> MASHHHHHHGSMAEGEEYDKILVLNFGSQYFHLIVKRLNNIKIFSETKDYGVELKDIKDMNIKGVILSGGPYSVTEAGSPHLKKEVFEYFLEKKIPIFGIAYGMQEIAVQMNGEVKKSKTSEYGCTDVNILRNDNINNITYCRNFGDSSSAMDL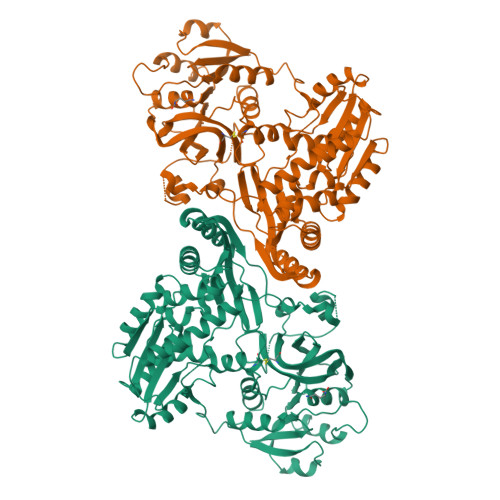YSNYKLMNETCCLFENIKSDITTVWMNHNDEVTKIPENFYLVSSSENCLICSIYNKEYNIYGVQYHPEVYESLDGELMFYNFAYNICKCKKQFDPIRYHELELKNIEKYKHDHYVIAAMSGGIDSTVAAAYTHKIFKERFFGIFIDNGLLRKNEAENVYTFLKSTFPDMNITKIDASENFLSNLQGVTDPEQKRKIIGKLFIEEFEKAVNNIDIDINKTFLLQGTLYPDIIESKCSKNLSDTIKTHHNVGGLPKNLKFKLFEPFKYLFKDDVKTLSRELNLPEEITNRHPFPGPGLAIRVIGEINKHKLNILREVDDIFINDLKQYGLYNQISQAFAVLLSSKSVGVRGDARSYDYVCVLRAVKTSSFMTANWYQIPYDILDKITTRILSEVKGVNRILYDVSSKPPATIEFE> GSHMDNQCTVQVRLELGHRAQLRKKPTTEGFTHDWMVFVRGPEQCDIQHFVEKVVFWLHDSFPKPRRVCKEPPYKVEESGYAGFIMPIEVHFKNKEEPRKVCFTYDLFLNLEGNLNHLRCEKLTFNNPTTEFRYKLLRAGGVMVMPEGAH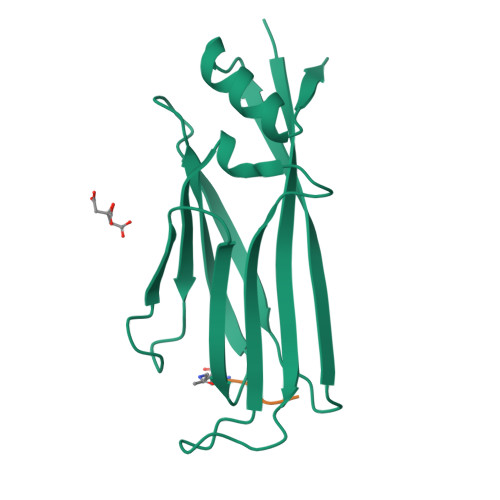HHHHH;> AARK[[(2R,3S,4R,5R)-5-(6-aminopurin-9-yl)-3,4-bis(oxidanyl)oxolan-2-yl]methoxy-oxidanyl-phosphoryl] 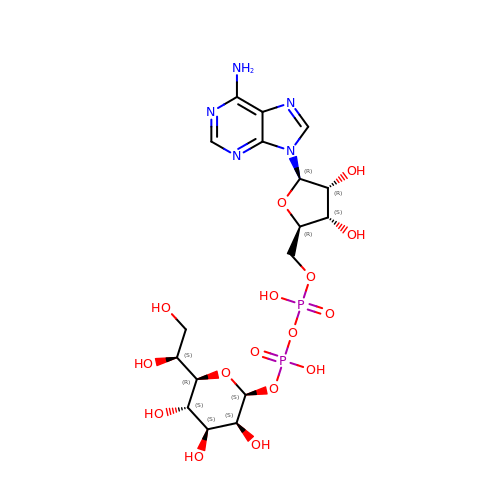[(2S,3S,4S,5S,6R)-6-[(1S)-1,2-bis(oxidanyl)ethyl]-3,4,5-tris(oxidanyl)oxan-2-yl] hydrogen phosphate | C17 H27 N5 O16 P2 | KMSFWBYFWSKGGR-DTBZDYEHSA-N>LGLQGGMLYPQESPSRECKELDGLWSFRADFSDNRRRGFEEQWYRRPLWESGPTVDMPVPSSFNDISQDWRLRHFVGWVWYEREVILPERWTQDLRTRVVLRIGSAHSYAIVWVNGVDTLEHEGGYLPFEADISNLVQVGPLPSRLRITIAINNTLTPTTLPPGTIQYLTDTSKYPKGYFVQNTYFDFFNYAGLQRSVLLYTTPTTYIDDITVTTSVEQDSGLVNYQISVKGSNLFKLEVRLLDAENKVVANGTGTQGQLKVPGVSLWWPYLMHERPAYLYSLEVQLTAQTSLGPVSDFYTLPVGIRTVAVTKSQFLINGKPFYFHGVNKHEDADIRGKGFDWPLLVKDFNLLRWLGANAFRTSHYPYAEEVMQMCDRYGIVVIDECPGVGLALPQFFNNVSLHHHMQVMEEVVRRDKNHPAVVMWSVANEPASHLESAGYYLKMVIAHTKSLDPSRPVTFVSNSNYAADKGAPYVDVICLNSYYSWYHDYGHLELIQLQLATQFENWYKKYQKPIIQSEYGAETIAGF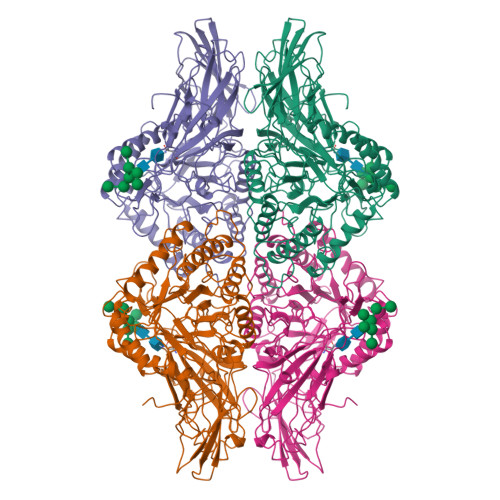HQDPPLMFTEEYQKSLLEQYHLGLDQKRRKYVVGELIWNFADFMTEQSPTRVLGNKKGIFTRQRQPKSAAFLLRERYWKIANET[2x]>MKNRNRMIVNGIVTSLICCSSLSALAASPPTEVKIVRDEYGMPHIYADDTYRLFYGYGYVVAQDRLFQMEMARRSTQGTVSEVLGKAFVSFDKDIRQNYWPDSIRAQIASLSAEDKSILQGYADGMNAWIDKVNASPDKLLPQQFSTFGFKPKHWEPFDVAMIFVGTMANRFSDSTSEIDNLALLTALKDKYGKQQGMAVFNQLKWLVNPSAPTTIAARESA[4x];>[4x]CNMWVIGKNKAQDAKAIMVNGPQFGWYAPAYTYGIGLHGAGYDVTGNTPFAYPGLVFGHNGTISWGSTAGFGDDVDIFAEKLSAEKPGYYQHNGEWVKMLSRKETIAVKDGQPETFTVWRTLHGNVIKTDTATQTAYAKARAWDGKEVASLLAWTHQMKAKNWPEWTQQAAKQALTINWYYADVNGNIGYVHTGAYPDRQPGHDPRLPVPGTGKWDWKGLLSFDLNPKVYNPQSGYIANWNNSPQKDYPASDLFAFLWGGADRVTEIDTTLDKQPRFTADQAWDVIRQTSRRDLNLRLFLPALKDATANLAENDPRRQLVDKLASWDGENLVNDDGKTYQQPGSAILNAWLTSMLKRTVVAAVPAPFGKWYSASGYETTQDGPTGSLNISVGAKILYEALQGDKSPIPQAVDLFGGKPQQEVILAALDDAWQTLSKRYGNDVTGWKTPAMALTFRANNFFGVPQAAAKEARHQAEYQNRGTENDMIVFSPTSGNRPVLAWDVVAPGQSGFIAPDGKADK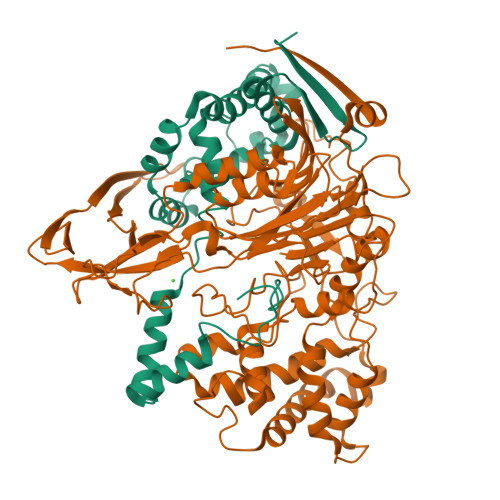HYDDQLIMYESFGRKSLWLTPQDVDEHKESQEVLQVQRLEHHHHHH Psychrophilic β-d-galactosidase from Arthrobacter sp. 32cB is an interesting candidate for industrial use, as it can hydrolyze lactose at rate comparable to mesophilic βDG from Kluyveromyces lactis. Furthermore, it exhibits additional transglycosylation activity, it catalyzes synthesis of GOS and HOS, for example: lactulose and alkyl glycosides. The functional dimer of ArthβDG has two independent active sites. Each of them is located on the top of TIM-barrel Domain 3 and is constituted of residues from both subunits of the dimer.

The question of the effect of point mutation of the other catalytic residue, E517, has not been answered before. As expected of the mutation of the catalytic residue, E517 into glutamine caused loss of function of the enzyme. The ArthβDG_E517Q exhibited no catalytic activity, whereas activity of mutant ArthβDG_D207A was severely depleted. Mutation of catalytic residue E517 into glutamine resulted in the elevation of the melting temperature of the mutant in respect to ArthβDG by 3.5–5 °C, depending on the investigated buffer solution. In the case of ArthβDG_E517Q, only a slight change in character of the active site was observed —similar to previously studied loss of function mutant ArthβDG_E441Q. Single-point mutations of residues E441 and E517 introduced in the enzyme’s active site were not sufficient to change spatial arrangement of galactosyl moiety bound in the deep binding mode but were enough to abolish the enzyme’s activity.

> EQMSVETPSALADSSPHTAPGSAGRSLELGAADIQDLESFEAGRGALPARAYLQSDAPRLSLNGEWQFRLSPGSRVAPDDGWQLGEALNGFESLPVPSSWPMHGHGAPAYTNVQFPFAVEPPHVPEANPIGDHLVVFEAGPEFFPHALLRFDGIESAGTVWLNGVELGTTRGSRLAHEFDVSGILEQGENTLAVRVAQFSAASYVEDQDMWWLPGIFRDVTLQARPAAGIDDVFVHAGYDHITGEGILKVEASRGGQAIDAVVRVPELALELAAGTEVRVPAVEPWSAEVPKLYEAAVSAAGESVALQIGFRSIAIEDAQFKVNGRRILLRGVNRHEHHPRLGRVVPRDVVEAELRLMKQHNINAIRTSHYPPHPQFLALADQLGFYVVLECDLETHGFESAGWAQNPSDDPQWEDALVDRMRRTVERDKNHASVVMWSLGNEAGTGRNLAAMSRWTKDRDPSRPIHYEGDWSSEHVDVYSRMYASQAETALIGQGIEPALNDAALDARRRAMPFVLCQYVHAMGNGPGGMSEYQALFEKYPRLMGGFVWEWLEHGITVSTADGVDHYGYGGDFGEEVHDGNFVTDGLVDADRRPRPGLLDFKKVIEPLRIDVARDWTGFTLRNGQDFADTSAFSFRYEVEADGGALDGGTVDVAPVAPQSETVVELPGSVAALAAGLSDGRPAVLTVRAVLGADSAWADAGHEVAWGQSVREPGAPVPPAPVEPVQVQDSELTLGPVVFSRATGMPTSIGGVPVEKLGLTLWWAPTDNDLGREWGGADERPLATQWKDAGLNRLHTRLLGISANPGQDGGETLTVRTRVSAADKQYGVLVDYTWSTDGETVGLRTQVRRDGTWVNRGFEVEWARIGLEFVLGEETELVSWFGQGPHQSYPDTGQGARAGWFSLPLAKMDVEYVRPQECGARSGSRSAALQLGGRTLEICGDPFALTVRPYSQDVLDAAAHRPDLKADGRTYLYVDHALRGVGTAACGPGVLEQYRLKPRDADFILTLKVRS>[2x]MSDPERRVRSTLKKVFGFDSFKTPLQESATMAVVKGNKDVFVCMPTGAGKSLCYQLPALLAKGITIVVSPLIALIQDQVDHLLTL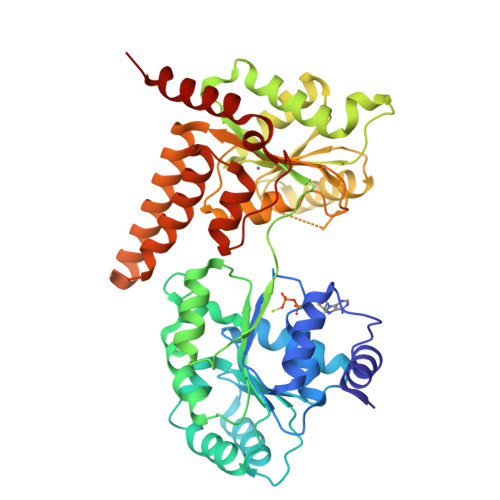KVRVSSLNSKLSAQERKELLADLEREKPQTKILYITPEMAASSSFQPTLNSLVSRHLLSYLVVDEAHCVSQWGHDFRPDYLRLGALRSRLGHAPCVALTATATPQVQEDVFAALHLKKPVAIFKTPCFRANLFYDVQFKELISDPYGNLKDFCLKALGQEADKGLSGCGIVYCRTREACEQLAIELSCRGVNAKAYHAGLKASERTLVQNDWMEEKVPVIVATISFGMGVDKANVRFVAHWNIAKSMAGYYQESGRAGRDGKPSWCRLYYSRNDRDQVSFLIRKEVAKLQEKRGNKASDKATIMAFDALVTFCEELGCRHAAIAKYFGDALPACAKGCDHCQNPTAVRRRLEALERSSSW Chaperonins are essential protein-folding machines, classified into three structural and phylogenetic groups: Group I (bacterial GroEL), Group II (archaeal thermosome and eukaryotic CCT), and Group III (bacterial thermosome-like). All chaperonin monomers share a common three-domain structure: an apical domain involved in substrate recognition, an equatorial domain containing the ATP-binding site that drives the conformational changes that occur during the chaperonin functional cycle, and an intermediate domain linking the two by relaying signals. Using ancestral sequence reconstruction (ASR) and protein resurrection, we inferred and experimentally characterized the last common ancestors of these groups (ancestral chaperonins ACI, ACII, and ACIII). We selected several AC nodes for protein synthesis and purification, including the last common ancestors of Group I (ACI), Group II (ACII), and Group III (ACIII), along with the ancestor of the Fibrobacteres–Chlorobi–Bacteroidetes (FCB) Group (AFCB).

ACII formed a heterogeneous mixture of eight-subunit oligomers, including both single and double rings, even without ATP. ACII was purified as a mixture of monomers and oligomers, and the presence of ATP triggered the typical conformational changes in chaperonins, transitioning between open and closed states. The 2D and 3D analysis of the particles revealed both single- and double-ring structures in both open and closed configurations. When comparing this structure with modern chaperonins such as E. coli GroEL (Group I) or the group II eukaryotic chaperonin CCT, we found that ACII possesses a built-in helical lid protrusion, similar to CCT. This feature allows ACII to close its cavity without needing a separate co-chaperonin like GroES, which GroEL requires. In ACII, a similar salt bridge exists between H299 and E334. However, due to a lack of interactions in the tip of the apical region, E334 forms a stronger interaction with K303. Altogether, these observations suggest that while ACII possesses a built-in lid that reduces reliance on a GroES-type cochaperonin for cavity closure, the resulting closure is less complete than that of CCT subunits, where total sealing prevents solute entry or exit. Despite its lack of detectable ATPase activity, ACII proved to be highly effective at protecting LDH from heat inactivation.

>[16x]MGQPMVVLSENTERTSGRDARKNNIAAARAIADMVKTTLGPRGMNKMLVNSLGDVTITNDGATILEEMDIEHPAAKMLKEVAKAQEEEAGDGTTTAVVLAGALLEEAEKLIEQGIHPTTIIKGYRKAVDKALEVLEEVAIPVDPDDEETLKAVARTAMTGKASEENREEIADLVVEAVLSLAEDGGGKYRVDLDNIKIEKQTGGGASDTELIEGVVLDKEPVHEDMPKKLENAKVAVLDAPIEVEKTELDAKISISSPEQFQAFLDQEEKQLREMVDKIVDTGANVVFCEKGIDDQVEHMLAKKGILAVRRVKKDDLEKIAKATGARVVSNIDELTPEDLGHAGLVEQRKKGEDRMVFVSGCKNEPVATILIRAATEHVVEELERAIDDALNAVKAAIKDGKVVPGGGAAEVAVARKLREYAKSLSGKEQLAIEAFADALEEIPRTLAENAGLDPIDTLVQLRAAHEEGDKNIGIDCLTGEVADMLEAGVIDPAAVKKQAIKSATEAATMILRIDDIIPAKAPTGEDGDG In mitosis, the augmin complex binds to spindle microtubules to recruit the γ-tubulin ring complex (γ-TuRC), the principal microtubule nucleator, for the formation of branched microtubules. The elongated structure of the augmin complex is characterised by extensive coiled-coil segments and comprises two structural elements with distinct but complementary functions in γ-TuRC and microtubule binding, linked by a flexible hinge. The augmin complex is recruited to microtubules via a composite microtubule binding site comprising a positively charged unordered extension and two calponin homology domains. By acting as an elongated structural scaffold, augmin positions the γ-TuRC on the pre-existing microtubule in a partially flexible manner, allowing the γ-TuRC to nucleate a branched microtubule in an approximate orientation with respect to the mother microtubule.

Aiming to validate the TIII models predicted by AlphaFold-Multimer using experimental approaches, we purified the X. laevis TIII tetramer24 after recombinant expression (HAUS1-EGFP-HIS8, 2xFLAG-HAUS3, HAUS4 and HAUS5) in insect cells. We next subjected the purified augmin TIII tetramer to cryo-EM single particle analysis, obtaining a cryo-EM reconstruction at 7.7 Å global resolution (and Methods section). Strikingly, the predicted TIII models provided an almost ideal fit into the cryo-EM reconstruction, explaining all resolved density segments on secondary structure level. We next optimised the fit of the highest-scoring model into the cryo-EM density by molecular dynamics flexible fitting (MDFF), which resulted in only minor adjustments. The overall elongated structure of the augmin TIII tetramer is characterised almost entirely by extensive coiled-coil segments that are predominantly formed in a pair-wise manner between HAUS3 – HAUS5 and HAUS1 – HAUS4, respectively. The TIII structure is characterised by a central ‘bulge’ region, composed of all four HAUS proteins, separating the TIII tetramer into two segments. While one of the two segments is assembled exclusively from the HAUS3 and HAUS5 subunits (H3/H5-arm), the other segment is formed by all four HAUS proteins (4H-arm). The N-terminal segments of all HAUS proteins are located in the bulge region, while their C-terminal segments form the 4H-arm. The very C-termini of HAUS1 and 4 are located at the tip of the 4H-arm and are predicted to form a flexible kinked coiled-coil. Cumulatively, integrating structural data from cryo-EM, crosslinking mass spectrometry and neural network-based structure prediction, we could in detail elucidate the structure and conformational plasticity of the augmin TIII tetramer, the functional module for γ-TuRC binding. These data indicate that the core segments of TIII form an overall rigid structural scaffold likely serving for specific binding and positioning of the γ-TuRC relative to the pre-existing microtubule.

> MDEKSTKIIMWLKKMFGDKPLPPYEVNTRTMEILYQLAEWNEARDKDLSLVTEDLKLKSAEVKAEAKYLQDLLTEGLGPSYTNLSRMGNNYLNQIVDSCLALELKNSSLSSYIPAVNDLSSELVAIELNNQEMEAELTSLRKKLTEALVLEKSLERDLKKAEEQCNFEKAKVEIRSQNMKKLKDKSEEYKYKIHAAKDQLSSAGMEEPLTHRSLVSLSETLTELKAQSMAAKEKLNSYLDLAPNPSLVKVKIEEAKRELKATEVELTTKVNMMEFVVPEPSKRRLK;> MSGGDRFVQTLQKLNYPKGAQLDGEDFDWLFEAVDLKPFLDWFCSAASEQNVVPDEKLQAFNTLKESGKPVLDEKALDEVLKTFSISKVPAIEEVAIEKLEEEVKALQKQKNLHIRRRNKLQMVESGNRQMCLKSKDKEEETGRAFQEVLHLLRVTNKKLNHELQSIVNGVQTLMSFFSTPETACELSSQPIFLSQLLLDKYLSLEEQSTAALTSFTKEHFFEGMSKFVEGSDENFQLVQLNVNSFGEDGTTEDKCKEMMRLQLAYICAKHKLIQMKAKSASLKVGLQWAENNASVVQDKASQKEENLKVRITSLKNETLQIENHTNSISNEKLPGLVRDNAQLLNMPIVKGDYDLQMAHQTSCSSRQDLVCDHLMKQKASFELLQLGYELELRKHRDVYRELGSIVQELKESGDKLEERLTMLSDVNLLSASKPRSNIDSKDLTSHRLYQLLDGDNTQKLFRTYDGLESVAQKLSQDIASMRDQLEVSEQEHSLLLSKLDSHLKELRDFMYPEGNTLMLTTPELSGEFHQLGSQLEKLNHITVEILGDLQLKRKMLESNKLQQIEKQLYVYFFQNEEQLKSIVGKLEAQTGGGSSA;> MAQTLQYVSSRLSMLQIDEEDLERNAQFGKVLIELCPLLGPNGGSANLNRELEETRRELLLQRKMWMRSEVIYQLVQEMLLDLQVRKLEGSLTEEERKFQDGLQQCMLVSECSRLLTADSVPPSDSTSILGLDKQDLLDLLPPNMLVLWVRDRLQKQLEEALKKKCFTFLSFHQPETDEEGDVLRAAKVLRLASTLEDEKRRLQNEQEKHQEMRALLEKQQEIYPHVLLRCLSLLRQAASELRLRAQSDIDRINAEYLEAKSNALFLKLRMEELQVLTDCYTPEKVLVHRQIRDTLEAGVKKEKQELSTSRQILSSYEFLGPEFEGLVQEYTRLKDKIKDNRWMLQELSKSLP;> MERRSLAQELKKWAVEEMGLPAQKAPSEEMLQRLFIGQCGDIWKFIIRHIHSHRTVRKIEGNLLWYQQLQHTEAQRTAEEEQQQRRKQLCKEILELRAELHHLQEQIQTAEREIVGQDLNCERAQDLCRRSLLLRAFNKKREEECEALCQSNKKIQYRCEQLQEIRRASQREVMFSAVDPDLSSSTFLEPEVLRDVREVCKLRFKFLRSLHDDSISSSVHPGKEDLRSLSHQQWMSMAEKVWNTHTPNHILAALERLTLNSTQELKKLQFSQAADLSKGPSCQLKEFSEPITQSRSCNESTHLDPQETLPSFHSLIQEGWANSVKVSSELRRVQSQAQALSEHLAERIQEIHKKLSDGSEVSVLTRAAFDAELRCVILRGCRDALMQECRMLQEEAAGKKQEMKLLQQQQQNIQEACLLLDKKQKHIQILIKGNSSSKSQIRRSSVEAQKYVQDKLLPWPQEIIQESQRLQDSIQKEVKHFSAICLPALLKVSTDGFNLLPSRELSINRMSNTHAPYYGIFKGIYESVRLPLYKAPESVLSHVADMKKQLFFLRSQLSSRSEAISKTQRALQKNTNPDTDALLKSLSDHYSLELDEMVPKMQRLIQQCEKHQEYGKEVQATVMDWWEQPVQLCLPSEERGGLTLRQWRERWTVAVTALQRATGSRS> MVPISPIETVPVKLKPGMDGPKVKQWPLTEEKIKALVEICTEMEKEGKISKIGPENPYNTPVFAIKKKDSTKWRKLVDFRELNKRTQDFWEVQLGIPHPAGLKKNKSVTVLDVGDAYFSVPLDEDFRKYTAFTIPSINNETPGIRYQYNVLPQGWKGSPAIFQSSMTKILEPFAAQNPDIVIYQYMDDLYVGSDLEIGQHRTKIEELRQHLLRWG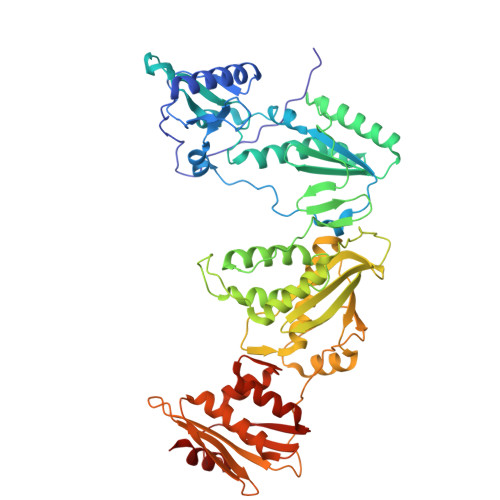LTTPDKKHQKEPPFLWMGYELHPDKWTVQPIVLPEKDSWTVNDIQKLVGKLNWASQIYPGIKVRQLSKLLRGTKALTEVIPLTEEAELELAENREILKEPVHGVYYDPSKDLIAEIQKQGQGQWTYQIYQEPFKNLKTGKYARMRGAHTNDVKQLTEAVQKITTESIVIWGKTPKFKLPIQKETWETWWTEYWQATWIPEWEFVNTPPLVKLWYQLEKEPIVGAETFYVDGAANRETKLGKAGYVTNKGRQKVVPLTNTTNQKTELQAIYLALQDSGLEVNIVTDSQYALGIIQAQPDKSESELVNQIIEQLIKKEKVYLAWVPAHKGIGGNEQVDKLVSAG>GPLGSKQARKDMALQHAVDLLEKMLADEEKKLTEFNLGDPLFESANDDPIKTLEEIIQEGDDVVGAHQLVVTQIKLRVQRNRRLADEIIREQLTDIRKVFSDKFEKLEQGIQNSYLLLDKLKTPFQDMRCLFEVANEQFNDTPVPPQYKEKFMVCLKQIVQYAVNSSSKLEKFVMLKIKTKKDDIKDRVTYTCMKYLLMAMQGTGGPKAINNEEHAKLFFKQLSNYDDLTDANHDGLELIKKLDKEQKEVAFHVNNFTHLVTTLGMALYKEGHQKNDEAMLGMHTPITMLSDQVRVLILYLIDEIVHAIHTNSNQSNDELIDGLKPKVRIVINEFHAT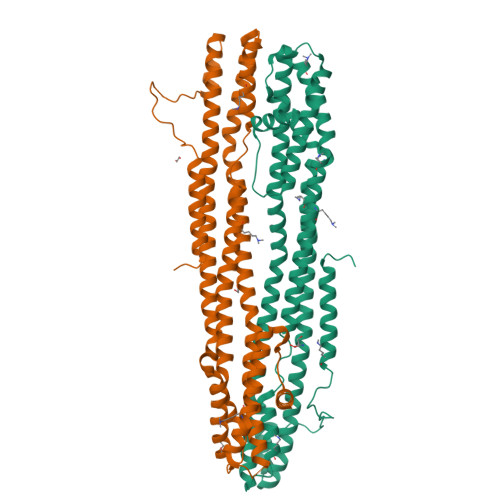LMMGIDKMKFYSLNELREIVNDKINED[2x]> 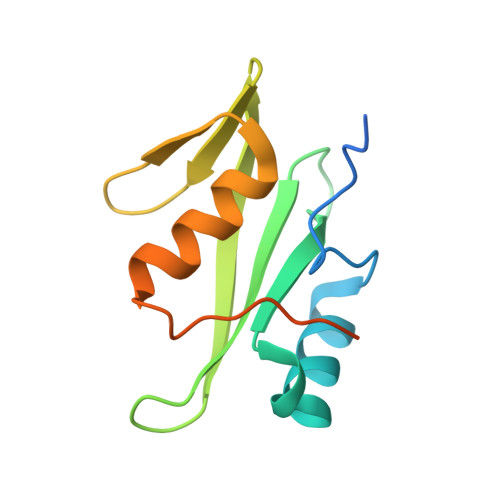GSGRAMDYVDVLNPMPACFYTVSRKEATEMLQKNPSLGNMILRPGSDSRNYSITIRQEIDIPRIKHYKVMSVGQNYTIELEKPVTLPNLFSVIDYFVKETRGNLRPFIASTDENTGQEPSMEGRS>[2x]GMSEPVFPTPEAAEDAFYAAFEARSLDDMMAVWARDDHVACIHPLAAPLNGRAAVAAGWRSMFGAAGRFRLQVKAVHEIRQADHVIRIVDEFLTIGD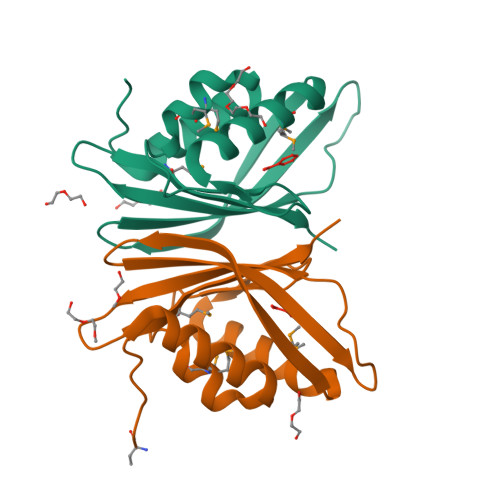ETAPRPAILATNVYRREADGWRMVLHHASPLQVGAKAGADTPPVVFH>MDKFRVQGPTRLQGEVTISGAKNAALPILFAALLAEEPVEIQNVPKLKDIDTTMKLLTQLGTKVERDGSVWIDASNVNNFSAPYDLVKTMRASIWALGPLVARFGQGQVSLPGGCAIGARPVDLHIFGLEKLGAEIKLEEGYVKASVNGRLKGAHIVMDKVSVGATVTIMSAATLAEGTTIIENAAREPEIVDTANFLVALGAKISGQGTDRITIEGVERLGGGVYRVLPDRIETGTFLVAAAISGGKIVCRNAQPDTLDAVLAKLREAGADIETGEDWISLDMHGKRPKAVTVRTAPHPAFPTAMQAQFTLLNLVAEGTGVITETIFENRFMHVPELIRMGAHAEIESNTVICHGVEKLSGAQVMATDLRASASLVLAGCIAEGTTVVDRIYHIDRGYERI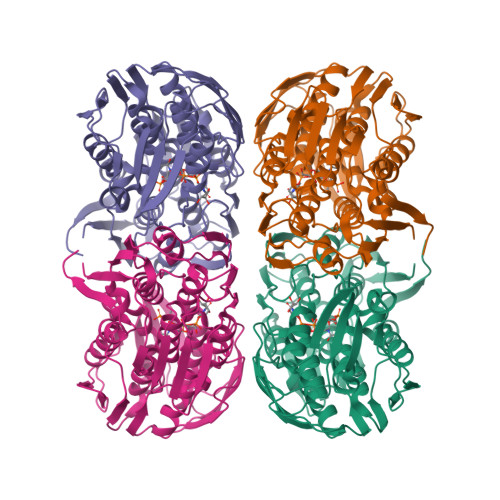EDKLRALGANIERVKGE[16x]> ELTQSRVQKIWVPVDHNSPTVIVMVGLPARGKTYISKKLTRYLNWIGVPTKVFNVGEYRREAVKQYSSYNFFRPDNEEAMKVRKQCALAALRDVKSYLAKEGGQIAVFDATNTTRERRHMILHFAKENDFKAFFIESVCDDPTVVASNIMEVKISSPDYKDCNSAEAMDDFMKRISCYEASYQPLDPDKCDRDLSLIKVIDVGRRFLVNRVQDHIQSRIVYYLMNIHVQPRTIYLCRHGENEHNLQGRIGGDSGLSSRGKKFASALSKFVEEQNLKDLRVWTSQLKSTIQTAEALRLPYEQWKALNEIDAGVCEELTYEEIRDTYPEEYALREQDKYYYRYPTGESYQDLVQRLEPVIMELERQENVLV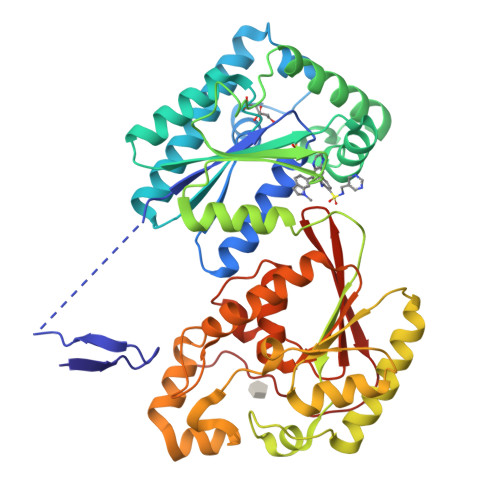ICHQAVLRCLLAYFLDKSAEEMPYLKCPLHTVLKLTPVAYGCRVESIYLNVESVCTHRERSE4,4'-[(3R,4R)-oxolane-3,4-diylbis(methylene)]bis(2-methoxyphenol) 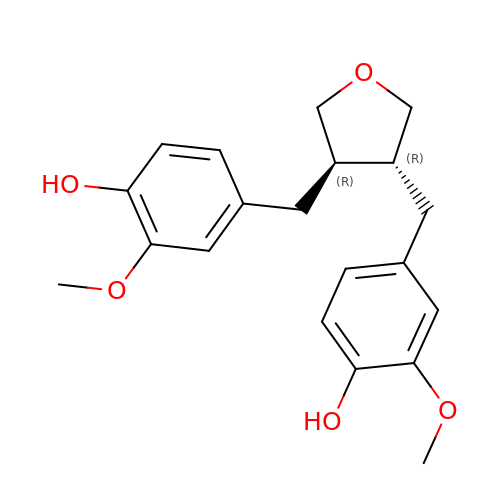| C20 H24 O5 | ROGUIJKVZZROIQ-HOTGVXAUSA-N>SPKKADYFKAKEVYNSSELIITQISENAFVHTSFKQTNDFGNVPCNGLVVKSNNEALVFDTPVNDKTSEELIKWINGTLHSKINAVVPTHFHDDSMGGLQAFHNHHIPSYAYSKTIELAKENNFTVPENNFKDSVVLKAGHKKAIAKFFGEGHTKDNVVGYLSEEHILFGGCLLKELEAGKGYLGDANVSAWSNTVEKVKKEYPDVKIVIPGHGEYGDQKLLDYTINLFKTQ[2x]

Here, we report the biochemical and structural characterization of two membrane-bound MBLs: CJO-1 and CIM-2, from Chryseobacterium joostei and Chryseobacterium indologenes, respectively. Both MBLs confer β-lactam resistance on producer bacterial strains and hydrolyze several antibiotics, although with impaired efficiency compared to NDM-1. The structures confirmed that both proteins adopt the characteristic αβ/βα sandwich fold of B1 subclass MBL enzymes (0.59 Å root mean square deviation [RMSD], over 220 Cα of CJO-1 with CIM-2), with two Zn(II) ions in their active sites (respectively). Specifically, a hindered access to the active site with the contribution of a Tyr residue in loop L10 and the presence of a positively charged Lys residue in loop L3 limit hydrolysis of cephalosporins with charged C3 substituents.

CIM-2, like the MBL CIM-1, was found in C. indologenes, an opportunistic pathogen of growing importance in the clinic which can express 19 variants of the soluble B1 MBL, IND-1, while CJO-1 was identified as a putative MBL sequence from the environmental organism C. joostei, first isolated in South Africa from dairy tanks. The sequences found for CJO-1 and CIM-2 were LLNC and ILSC, where the cysteine (C) residue is present at positions 16 and 20, respectively. Pairwise alignments reveal that CJO-1 and NDM-1 share a 25.1% sequence identity, while CIM-2 showed a 23.9% sequence identity with NDM-1 and 74.6% with CJO-1. Aiming to understand the substrate profile of these enzymes, we crystallized both CJO-1 and CIM-2 in their soluble forms and solved their X-ray structures using single wavelength anomalous dispersion (SAD) from data collected at the Zn edge. CIM-2 diffraction data extended to 1.56 Å resolution, and CJO-1 to 1.34 Å. CJO-1 and CIM-2 have the same conserved active site residues coordinating Zn1 (His116, His118 and His196) and Zn2 (Asp120, Cys221 and His263), and so have highly similar active site architectures, with similarity extending to the positioning of their active site water molecules. Loop L10 adopts similar conformations in CJO-1 and CIM-2, which are distinct from its conformation in the NDM-1 crystal structure, likely due to the presence of an extra amino acid in this loop in NDM-1, and further differences in amino acid sequence. Indeed, Asn233, present in NDM-1 and in most B1 MBLs, and previously proposed to interact with the carbonyl group of the β-lactam substrate, is substituted by a Tyr in CJO-1 and CIM-2, as observed in some other B1 MBLs such as BlaB and SPM-1 (34), and in all characterized B1 MBLs from Chryseobacterium spp.. Reflecting this flexibility, overall conformations of L3 differ between NDM-1 and CJO-1/CIM-2, and between CJO-1 and CIM-2, despite their high sequence identity in this region. However, Met61 and Trp87, which are part of a hydrophobic patch in NDM-1 and have been observed to be important for binding some inhibitors, are not conserved in CJO-1 (Thr61 and Thr87) or CIM-2 (Thr61 and Val 87).>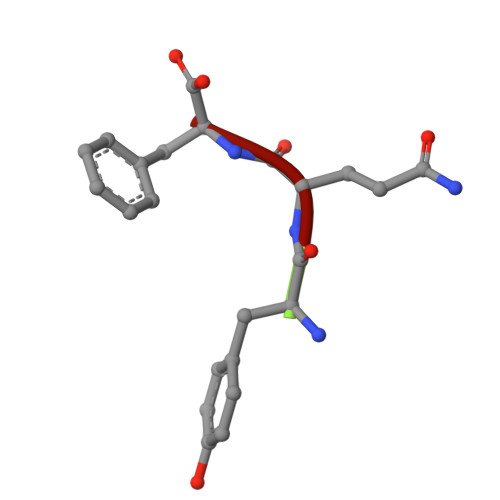 YQF> MAIVETVIDGINYFLSLSVTQQISILLGVPFVYNLVWQYLYSLRKDRAPLVFYWIPWFGSAASYGQQPYEFFESCRQKYGDVFSFMLLGKIMTVYLGPKGHEFVFNAKLSDVSAEDAYKHLTTPVFGKGVIYDCPNSRLMEQKKFAKFALTTDSFKRYVPKIREEILNYFVTDESFKLKEKTHGVANVMKTQPEITIFTASRSLFGDEMRRIFDRSFAQLYSDLDKGFTPINFVFPNLPLPHYWRRDAAQKKISATYMKEIKSRRERGDIDPNRDLIDSLLIHSTYKDGVKMTDQEIANLLIGILMGGQHTSASTSAWFLLHLGEKPHLQDV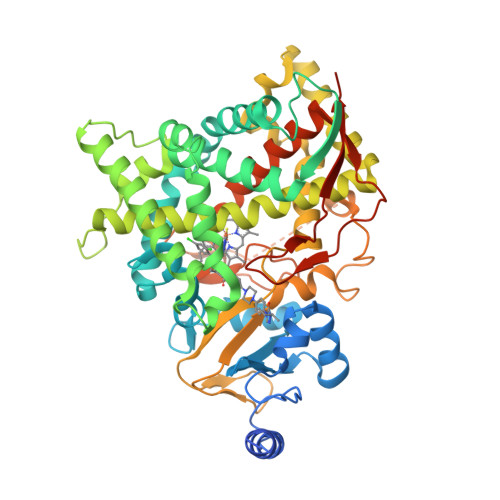IYQEVVELLKEKGGDLNDLTYEDLQKLPSVNNTIKETLRMHMPLHSIFRKVTNPLRIPETNYIVPKGHYVLVSPGYAHTSERYFDNPEDFDPTRWDTAAAKANSVSFNSSDEVDYGFGKVSKGVSSPYLPFGGGRHRCIGEQFAYVQLGTILTTFVYNLRWTIDGYKVPDPDYSSMVVLPTEPAEIIWEKRETCMFGGRHHHHHH>MKIKQVHVRASKIKLKETFTIALGTIESADSAIVEIETEEGLVGYGEGGPGIFITGETLAGTLETIELFGQAIIGLNPFNIEKIHEVMDKISAFAPAAKAAIDIACYDLMGQKAQLPLYQLLGGYDNQVITDITLGIDEPNVMAQKAVEKVKLGFDTLKIKVGTGIEADIARVKAIREAVGFDIKLRLDANQAWTPKDAVKAIQALADYQIELVEQPVKRRDLEGLKYVTSQVNTTIMADESCFDAQDALELVKKG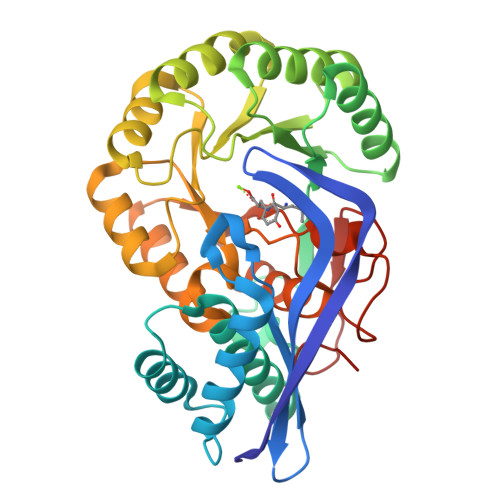TVDVINIKLMKCGGIHEALKINQICETAGIECMIGCMAEETTIGITAAAHLAAAQKNITRADLDATFGLETAPVTGGVSLEAKPLLELGEAAGLGISH[8x]(6-phenylpyridin-3-yl)methanamine | C12 H12 N2 | 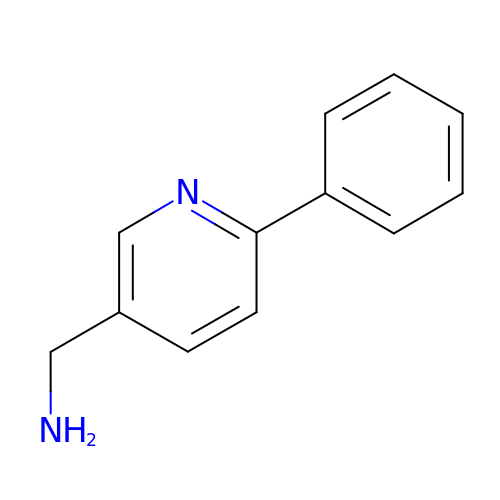YXWLMYSYKQXBQE-UHFFFAOYSA-N N-{(1S,2R)-1-(3,5-DIFLUOROBENZYL)-2-HYDROXY-2-[(2R,4R)-4-PHENOXYPYRROLIDIN-2-YL]ETHYL}-3-{[(2R)-2-(METHOXYMETHYL)PYRROLIDIN-1-YL]CARBONYL}-5-METHYLBENZAMIDE 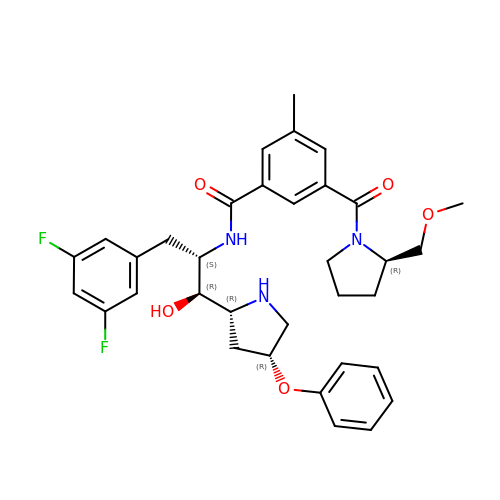| C34 H39 F2 N3 O5 | KYHYNSQLYDXSNK-MXWGZHRFSA-N> MKIERPMERRFSQPGKQISNTIKQLSNLPEEELPTYLNNIYEWRCAKTDLLYWVDVLDRFDEILKAVVTEYGLGQFQNKPMKESDKEMVYAILKFQKLLVENSSNKSMFSSFDVVEPFIYSFELDLAIEALYLVSFFASKIHIQRSIKTSMALMKMETLKTLIERVKEKPQSMYTYYDETTNNCKRVSIKKAVKKGIYSISDKMLPSQEIRRFIHAIRLHEMAEQHEKLKIIRMLAFSALVYYNYTDLPIDSEFISRDLPETLAIINTESYQMREAAVTMIDAIFRMRIRHSAVIAAMNAQSHEGMIMNLLKKVVNEDVPEHFAIVFFNFLSSCFASGPCVSALFSAGIVQYVCNTLRDQPDISYRKRMRLVMGANTFLFTLPAPFTWFISENGIRILSKELLLAVDVALGNIKDHDLLMYINSIMKIISQLFKNAGTAEAMRGFLEGEFPRAISLILFHSEEFTPSILAYLFSAVGDYIHNEPSNLPFIIEAGIFDGFVMCMKKELPESPDFLLELPNLIEAFFLNSELIKKIDEENILDRIFESFEIVNLSNIILMYDIGRAYGIFLENLVRHYPIISLTVKEKIYNTMKNLESMIPNTDPELMRLLLGNLFRMMHRAVYRKTTNNQLITDKGLLNNRIISMLMLIEIPTETELYTDVMNILMEVFDEDQTYVISYIAKVIDRVMKNKVTLENIEKIKRILLIVNYLIFKNEETCEEFIKHCTSKGFLQIVKRISQYFDNLKKDTALVSVAKNESLTNLYYSFTMGILKTVYRYSKTNAKEYLKIFGLLVEDLLSKTEQIDHLYYTQRMHGLKNYIMVDKSPQQYPQKNEFVVTQEYLMGINLSETLMEHAKNSVSMLKDEKITMDAHKKVVSSILEVLSIYVRGIKNLFVPVKEPKKKVCEIEEHVLIIVELLMDYIDKSSIEHLLNIVKTAFFVTLRKQITKEMDRENEGSAEYKRRNILGSFFISVFLNLPKEETEAVLKSDIFTILVKNKKTFKQVYNKNCFGLLQYAAIKESRVFSHLVSFIPKMTKQVGASTDPAFLKLYAVGLVFVAMRDTLKKTTVLSRFIGNIVFAESTCPAVVEAQGIVILAIVKLKIEYNLAITIEDPIIHLNRIYAIVETAEQKEGLVILANLLIRRVIESKEAAKEAVDTIIKNKHLGKSRMYTVHTVCSNLRNALFYSISSFLEYLSSNFECISAGWEEIRHKLPDESANPTESGQISEAVLETLSDGLFTKQIKIYSGLNAELFRTLFVHRATGKMEQIVRIHSLCLLVVSFPQLISTLVPEDYSFFMYFLENHAAYSKSLKPSAFQQEDKTLAYWSGHFIMLIFNHTTYVEVKKYILEKVLELLPT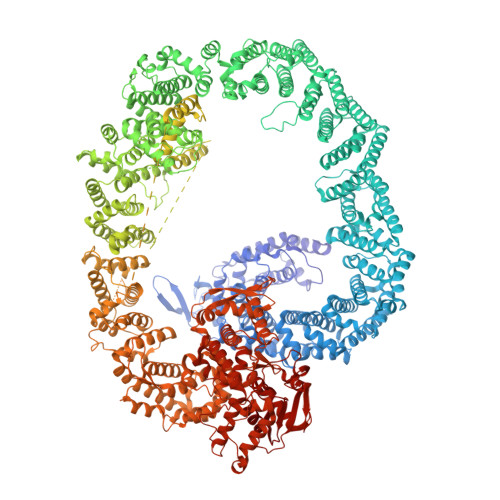SINATVIFSELIQEILTMRFSKNTFDENTALVKEMNCLEVMIRSTMQIDNRRKDYGSIMEILTKPMEYITRILAVDEKEAFYEEVTQSEEEVYFEDIDEGYMEDFDTDETMDSDQVVYDDTEENSQEVGELCSEDSLTVYTAESNNYGEYLMSDEESSSEEEGMDEEQSSSEQSEKNEFLKSLCILPISKLIGKEMEIFNADERMPFVQKILEGSIISNLQEKEPSSTDEETFDSEEGSYRRHQYLMRREEENDDEELNDYAIDPTDPDAHLDDEGPEEIDEGVDEYDDESQYDYDGNGSDDEEYDDEESFATGEEIAIGDENGEIPELDVEVLNNLPSSILEDTVENFYQDRISSSTEYRAISLHFLNRLREEVRSVFEEHEARYMETFAGEIVPRREEKKKKPQEMPFIAEREAAASVPIDIVFGLIHMVLQCGNRRNLYRIIHNISANKEVRIFSVETLVNSIYQAVVEGASSSAGAGSSTVNASAGSSGNNEVIAPEVITKRGFEALTYLCTKSSDFTTVFSYNTELINKILQATNKRTISESVKLLSTVGDCFNNDKVAEPENIEVRKYIGFLEYDMTDDTFKHFCEFIKKTDRFYRPMYLLYLMGGSKKSLEECLDKKAEFNSHTHHKGIIKLVRMLSLVNIMGITETYLDSLMELREMPFWEYYFNIILPKEKESLYASSILPLFKAFVIVHTIQMYIGRNENINEFSEIPNSDSSIYYSVVEKEKDLINTFIQADPDLLFHAFAGLQKKILDFDNKRIYFYKKIREDVQLRPTISLMVQRGAVFEDTFHQLMRLNGEQVRNAKFNIKFAGEEGVDAGGLTREWYSELSKEMFNANYALFTPIGSSYQPNHISHINPEHLVYFKFIGRIIGKAVYDEMTVDCHFTRAFYKRVLSIPVDLTDVEALDPEFHRSLVWILENDIENVLDMTFSIEQDRFGITEIIDLKENGRNIAVTNENKREYVELVCRFKLVRVIERQLSAFAEGFFEILDVDMLKMFNEKELELLISGLPEIDVDDWRNNTIYFGYTSDSQVIRWYWRAVRNFSMEERAKLLQFATGTSKLPLEGFAGLRCQNGNQKFQIHKASGGSSRLPTAHTCFNQLDLPEYDSYEQLVKALLFSLEECTSGFGFA> MPLPIPSLL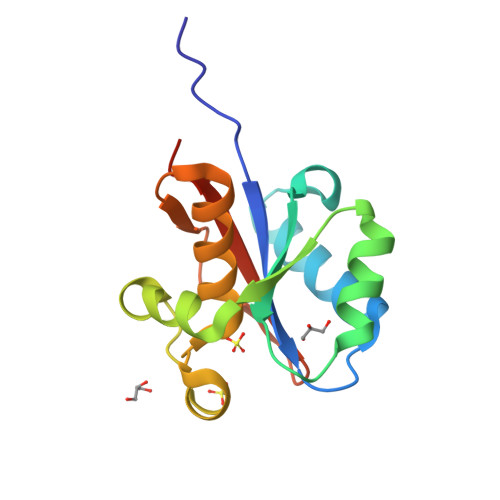IAGIGSRRGCSAEHLRALLERTLGEHGRSLAELDALASIDGKRDEPGLRQLATLLERPVHFLAPAVLHDYEPRLLSPSAVALRETGCSSVAEAAALALAERLGGGRADLLGAKRSDDRASIALARLLTERELP>MSKDTEDSRKIWRTIMLLLVFAILLSAIIWYQITTNPDTSQIATLLSMQLLLIALMLVVIALLLSRQTEQVAESIRRDVSALAYVMLGLLLSLLNRLSLAAEAYKKAIELDPNDALAWLLLGSVLEKLKRLDEAAEAYKKAIELKPNDASAWKELGKVLEKLGRLDEAAEAYKKAIE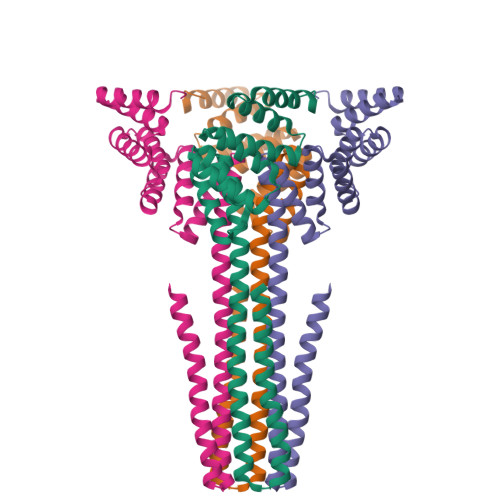LDPEDAEAWKELGKVLEKLGRLDEAAEAYKKAIELDPNDLEHHHHH[4x]>MSNNIKHETDYSHDWTVEPNGGVTEVDSKHTPIIPEVGRSVDIENTGRGELTIQYQWGAPFMAGGWKVAKSHVVQRDETYHLQRPDNAFYHQRIVVINNGASRG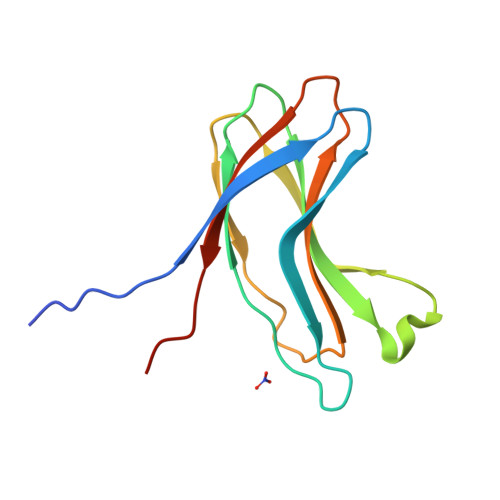FCTIYYHLEHHHHHH[2x]>[12x]LATTSDHDFSYLSFAYDATDLELEGSYDYVIVGGGTSGCPLAATLSEKYKVLVLERGTLPTAYPNLLTSDGFIYNLQQEDDGQTPVERFVSGDGIDDVRGRVLGGTSMINAGVYARANTKIFSASGIEWDMDLVNQTYDWVEDTIVYKPDKQAWQSLTKTAFLEAGVLPDNGFSLDHEAGTRLTGSTFDNNGTRHASDELLNKGDPNNLRVAVHASVEKIIFSSNSSGVTAIGVIYKDSN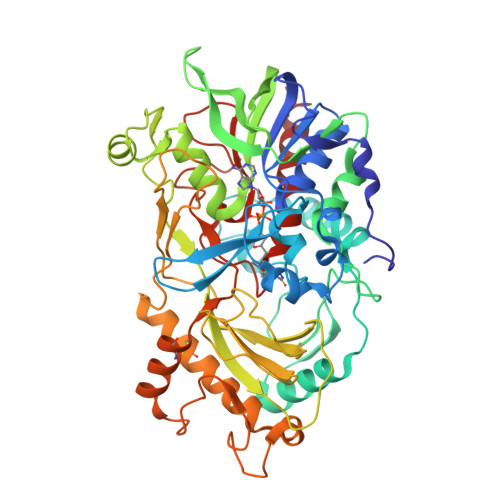GTPHQAFVRGEGEVIVSAGPIGSPQLLLLSGVGPESYLSSLNIPVVLSHPYVGQFLHDNPRNFINILPPNPIEPSTVTVLGITSNFYQCSFSSLPFSIPPFAFFPNPTYPLPNSTFAHFVNKVPGPLSYGSITLNSDSDVRVAPNVKFNYYSNSTDLAHCVSGMKKIGELLSSDALKPYKVEDLPGIDGFDILGIPLPENQTDDAAFETFCREAVASYWHYHGGCLVGEVLDGDFRVTGINALRVVDGSTFPYSPASHPQGFYLMLGRYVGSKILQERSAA> ELYPLA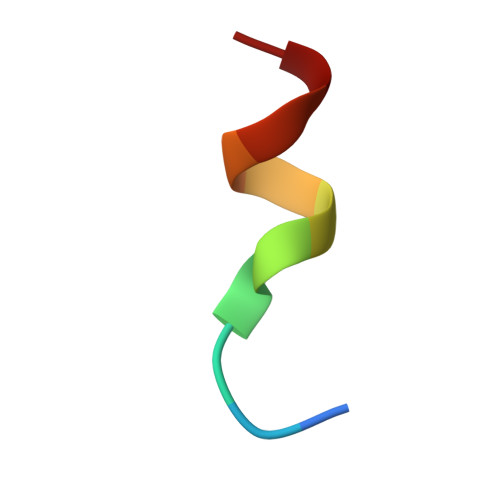SLRSL>[2x]APRKFFVGGNWKMNGDKKSLGELIHTLNGAKLSADTEVVCGAPSIYLDFA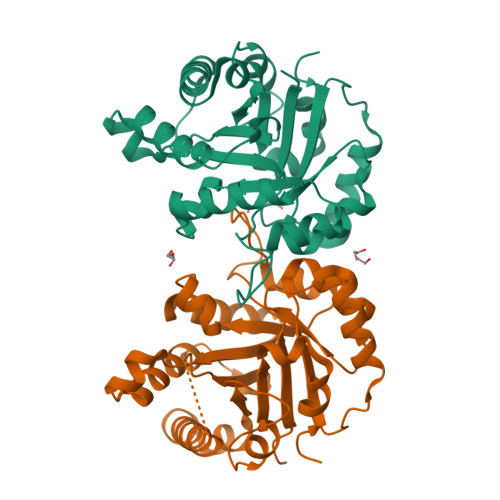RQKLDAKIGVAAQNCYKVPKGAFTGEISPAMIKDIGAAWVILGHSERRHVFGESDELIGQKVAHALAEGLGVIACIGEKLDEREAGITEKVVFEQTKAIADNVKDWSKVVLAYEPVWAIGTGKTKTPQQAQEVHEKLRGWLKSHVSDAVAQSTRIIYGGSVTGGNCKELASQHDVDGFLVGGASLKPEFVDIINAKH> MLDRFATKQTQEKLKIGVVGTFAIGCLFPLLSDFKRSYPHIDLHISTHNNRVDPAAEGLDYTIRYGGGAW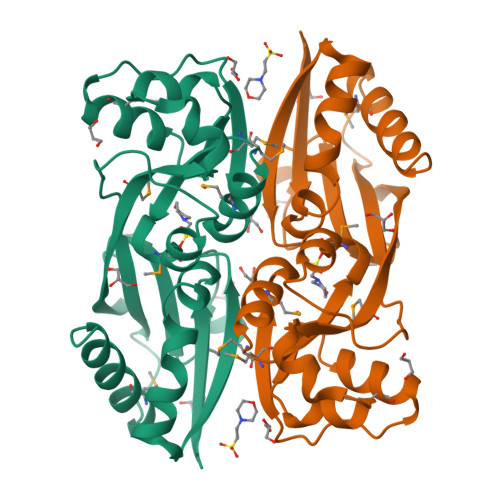HDTDAQYLCSALMSPLCSPTLASQIQTPADILKFPLLRSYRRDEWALWMQTVGEAPPSPTHNVMVFDSSVTMLEAAQAGMGVAIAPVRMFTHLLSSERIVQPFLTQIDLGSYWITRLQSRPETPAMREFSRWLTGVLHKTSGSHHHHHH> SSYMEQEEDWDRDLLLDPAWEKQQRKTFTAWCNSHLRKAGTQIENIEEDFRNGLKLMLLLEVISGERLPRPDKGKMRFHKIANVNKALDFIASKGVKLVSIGAEEIVDGNLKMTLGMIWTIILRFAIQDISVEETSAKEGLLLWCQRKTAPYRNVNVQNFHTSWKDGLALCALIHR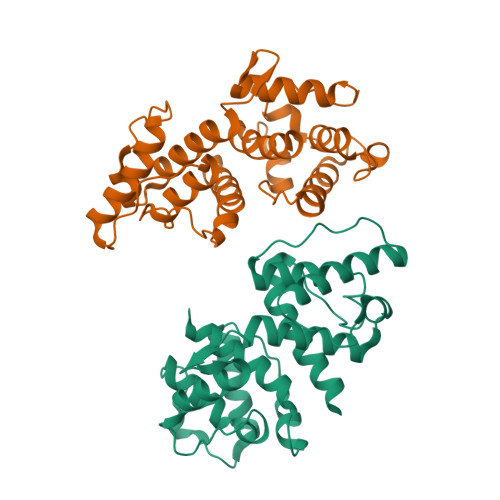HRPDLIDYAKLRKDDPIGNLNTAFEVAEKYLDIPKMLDAEDIVNTPKPDEKAIMTYVSCFYHAFAGAEQAETAA Members of glycosyltransferase family 75 (GT75) not only reversibly catalyze the autoglycosylation of a conserved arginine residue with specific NDP-sugars but also exhibit NDP-pyranose mutase activity that reversibly converts specific NDP-pyranose to NDP-furanose. MtdL from deep sea–derived Marinactinospora thermotolerans SCSIO 00652 has been discovered in the antibiotic A201A biosynthetic pathway, generating GDP-L-galactofuranose (L-Galf) from GDP-L-galactopyranose (L-Galp). The MtdL subunit is divided into three regions: the N-terminal region (residues 1–111), the core region (residues 112–291), and the C-terminal region (residues 292–376). The characteristic DXD motif (Asp109-Asp110-Asp111), together with conserved His287, coordinates a Mn2+ ion, which stabilizes the diphosphate of the nucleotide.

We also obtained crystal structures of the catalytically deficient S228A mutant of MtdL in complex with GDP-L-Fucp·Mn2+ and GDP-L-Fucf·Mn2+, respectively, and the R257K mutant bound with Mn2+. Arg257 directly hydrogen bonds to the β-phosphate. Moreover, Arg257 interacts with both the sugar and the β-phosphate moieties of the substrate. It is a critical substrate-binding residue since no electron density was observed whether for the GDP or for the D-Glcp moiety in the structure of MtdL-R257K·Mn2+ cocrystallized with GDP-D-Glcp, consistent with abrogated mutase activity of R257K. Because Asp109, Gln229, and Arg257 interact with both the GDP and the sugar moieties, the almost abrogated mutase activity of the D109N, Q229A, and R257K mutants might be due to significantly decreased binding of these mutants to GDP-sugar substrate.

>[2x]HMSGRDISTAVVVTTISDGGFLDRLAPALRDAGARLIVIPDRNTGPALFAACERHRRLGLDVVCPSVAEQQDLLERLAVPDLIPYHSDNRRNVGYLMAWMEGFDVIVSMDDDNLPTTDDFVERHQVVCQGPRTQPVTASSDGWFNNCALLEVEPTEVFPRGFPFHARPAHAQARTSVCERPADVRINAGLWLGDPDVDAITRLAVRPNALAHSGGSVVLAEGTWCPVNSQNTAVHRDALPAYYFLRMGQPVDGVPMEKFGDIFSGYFVQVCAQHLGHAVRFGDPVVEHPRNEHDLLDDLHKEVPAVRLLDDILDHLRDHPLEGGDYLETYESLSYALQEIAERVNGRAWSPDARAFLHRSAHLMRSWTGALRTVAGT> MTKSRKQKQKKQDFLRKKLKVGKPKEKARNATDTSFVSKTISIRNQHLDQNPHDLTKRLTLLKHHNINVRKETLTTFQKSIPSIIKSRLMTPLLTQSIPLICDESQQVRQGLIDLVDEIGSHDAEILKLHCNIFVLYINMAMTHIVTQIQADSTKFLSHLLKYCGDEVVRKSWVKLLNGVFGVLGWGQVGKNDSASIVQTKKRNAKYVTIHLNALYTLVEYGCQDERARSDGDTAETTEDSGTLRNPYLIPDYPQPFEHLKLFTREL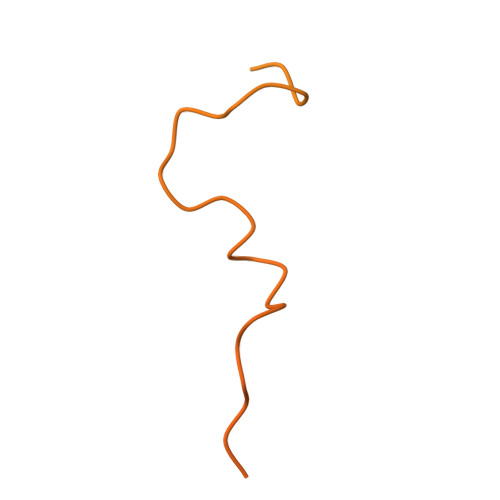KVQDATSSGVNATLLSLATQDIDTRKAVFIEQFLPIVRKKIEVIIKEGGECGKSANKLKTLLAKIFD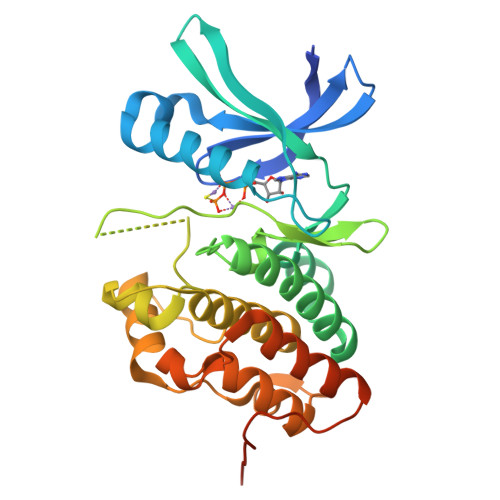>[4x]GSHMTTPSHLSDRYELGEILGFGGMSEVHLARDLRDHRDVAVKVLRADLARDPSFYLRFRREAQNAAALNHPAIVAVYDTGEAETPAGPLPYIVMEYVDGVTLRDIVHTEGPMTPKRAIEVIADACQALNFSHQNGIIHRDVKPANIMISATNAVKVMDFGIARAIADSGNSVTQTAAVIGTAQYLSPEQARGDSVDARSDVYSLGCVLYEVLTGEPPFTGDSPVSVAYQHVREDPIPPSARHEGLSADLDAVVLKALAKNPENRYQTAAEMRADLVRVHNGEPPEAPKVLTDAERTSLLSSAAGNLSGPR>EATLGSGNLRQAVMLPEGEDLNEWIAVNTVDFFNQINMLYGTITEFCTEASCPVMSAGPRYEYHWADGTNIKKPIKCSAPKYIDYLMTWVQDQLDDETLFPSKIGVPFPKNFMSVAKTILKRLFRVYAHIYHQHFDSVMQLQEEAHLNT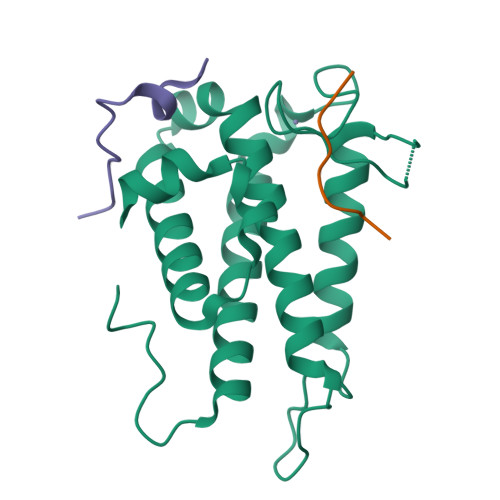SFKHFIFFVQEFNLIDRRELAPLQELIEKLGSKDR[2x];>[4x]ALPAWARPDYNPPLVESWRR>[4x]MASKEEDNMASLPKTHELHIFGSFNGVKFDMVGEGTGNPNEGSEELKLKSTNGPLKFSPYILVPHLGXAFYQYLPFPDGMSPF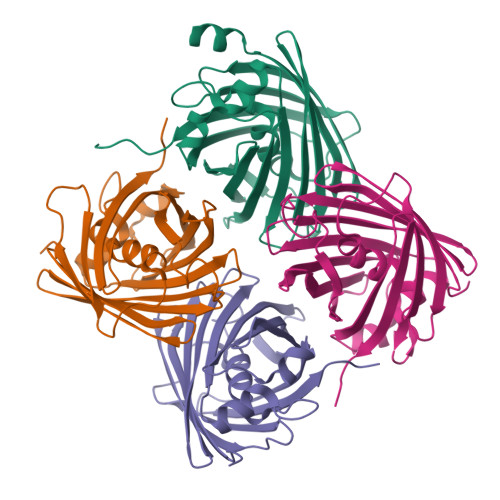QAAMHDGSGYQVHRTIQYEDGASVTAHYRYTYEGSHIKGEFQVIGTGFPPDGPVMTNKLTAMDWHVTKMLYPNDKTILSTADISYTTTAGKRYQSKMRENNTFAKPMAADILQKQPMFVFRKSELQHSKTELTFKEWQKAFTDVMSGGSHHHHHH>[2x]QRTCLICGDRATGLHYGIISCEGCKGFFKRSISN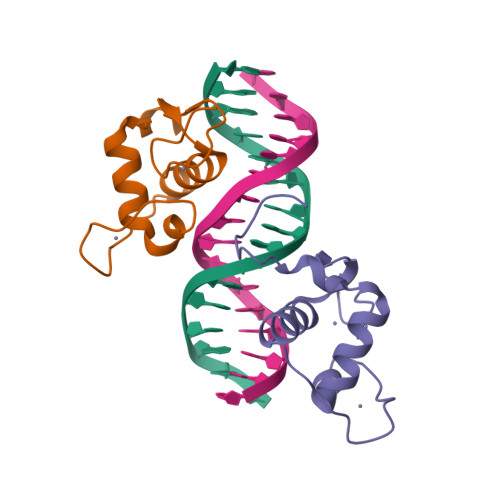KRVYRCSRDKNCVMSRKQRNRCQYCRLLKCLQMGMNRKAIREDGMPGGRN>[2x]XRMKQIEDKIEEIESKQKKIENEIARIKKLLQLTVWG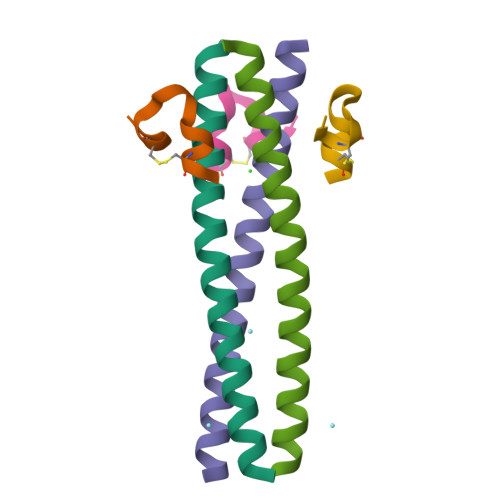IKQLQARILX;>[2x]XKKGACESPEWQWLCAAX> MLAKDKVALLIGNMNYREHPKLKAPLVDVYELTNLLRQLDFKVVSLLDLTEY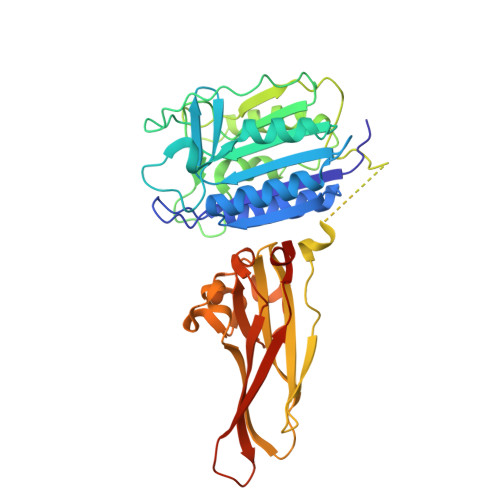EMRNAVDEFLLLLDKGVYGLLYYAGHGYENFGNSFMVPVDAPNPYRSENCLCVQNILKLMQEKETGLNVFLLDMCRKRNDYDDTIPILDALKVTANIVFGYATCQGAEAFEIQHSGLANGIFMKFLKDRLLEDKKITVLLDEVAEDMGKCHLTKGKQALEIRSSLSEKRALTDPIQGTEYSAESLVRNLQWAKAHELPESMCLKFDCGVQIQLGFAAEFSNVMIIYTSIVYKPPEIIMCDAYVTDFPLDLDIDPKDANKGTPEETGSYLVSKDLPKHCLYTRLSSLQKLKEHLVFTVCLSYQYSGLEDTVEDKQEVNVGKPLIAKLDMHRLEHHHHHH>[2x]MGSSHHHHHHSSGLVPRGSHMASMESTLGWSVQDWLSFHSKSTPTKSLELLENLLKSQKPAPEDPAWISLIPVEDLHHQWNILQSKSNKEELPLYGVPIAVKDNIDYKGLPTTAACPSYLYQPTRDSYVVELLRDAGAVVIGKTNLDQFATGLVGTRSPYGKTPCVFNDKYVSGGSSAGSASVVGRGIVPLSLGTDTAGAGRVPAALNNLIGLKPTKGAFSCRGVVPACKSLDCVSVFALNLSDAEIAFKVMNKPDLLEDEYSREFPKNPISQYPKDLTIAIPKEVPWFGETENPKLYTKAVASLKNTGAKIVVVDFEPLLELARCLYEGAWVAERYCATRDFLATNPPESSLDETVVNIIKGAVKFDAADAFKFEYKRQGILQKVNLLLKDIDVLCVPTCPLNPKLEEVAQEPVLVNSR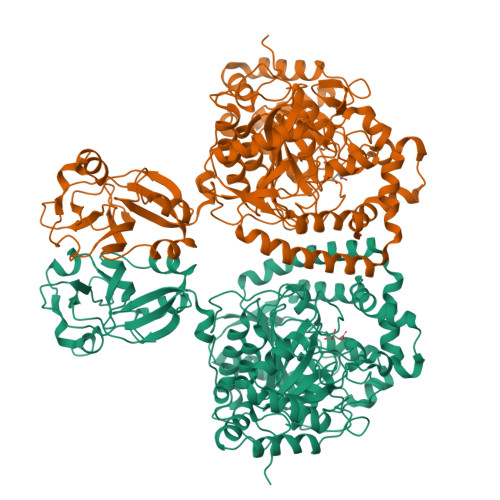QGTWTNFVNLADLAALAVPSGFRSDGLPNGITLIGKKFSDYALLDLAKRFFSVAFPNNSRTYGKFVDRRITVEDELDGPSKDTLNGVKLAVVGAHLKGLPLHWQLQKCNATYLSSPKTSNNYKLYALPKVGPVLKPGLRRVNDGTGSQIQLEVYSVPYDRFGDFIAMVPEPLGIGSVELESGEWVKSFICEEFGYTQQGTVDITKFGGFKPYIEHIQVTEAQKK>[2x]MFRLEDFNFHNKTVFLRVDLNSPMKDGKIISDARFKAVLPTIRYLIESGAKVVIGTHQGKPYSEDYTTTEEHARVLSELLDQHVEYIEDIFGRYAREKIKELKSGEVAILENLRFSAEEVKNKPIEECEKTFLVKKLSKVIDYVVNDAFATAHRSQPSLVGFARIKPMIMGFLMEKEIEALMRAYYSKDSPKIYVLGGAKVEDSLKVVENVLRRERADLVLTGGLVANVFTLAKGFDLGRKNV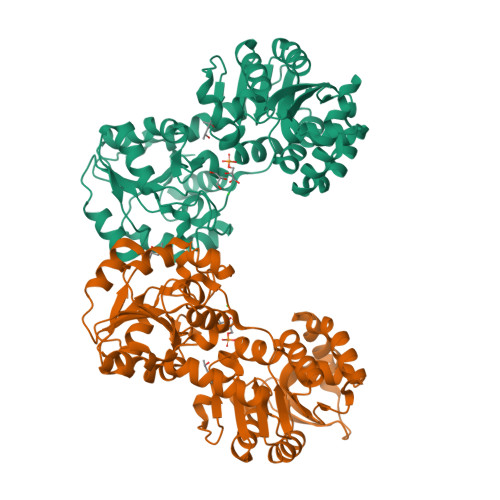EFMKKKGLLDYVKHAEEILDEFYPYIRTPVDFAVDYKGERVEIDLLSENRGLLHQYQIMDIGKRTAEKYREILMKARIIVANGPMGVFEREEFAIGTVEVFKAIADSPAFSVLGGGHSIASIQKYGITGITHISTGGGAMLSFFAGEELPVLRALQISYEKFKEVVK> GEGQQHHLGG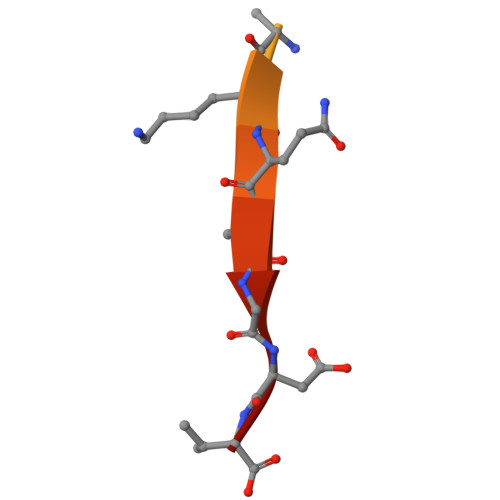AKQAGDV>[2x]GSMELRVGNRYRLGRKIGSGSFGDIYLGTDIAAGEEVAIKLECVKTKHPQLHIESKIYKMMQGGVGIPTIRWCGAEGDYNVMVMELLGPSLEDLFNFCSRKFSLKTVLLLADQMISRIEYIHSKNFIHRDVKPDNFLMGLGKKGNLVYIIDFGLAKKYRDARTHQHIPYRENKNLTGTARYASINTHLGIEQSRRDDLESLGYVLMYFNLGSLPWQGLKAAT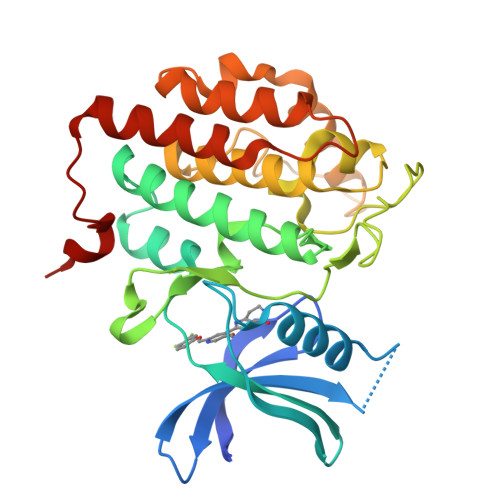KRQKYERISEKKMSTPIEVLCKGYPSEFATYLNFCRSLRFDDKPDYSYLRQLFRNLFHRQGFSYDYVFDWNMLK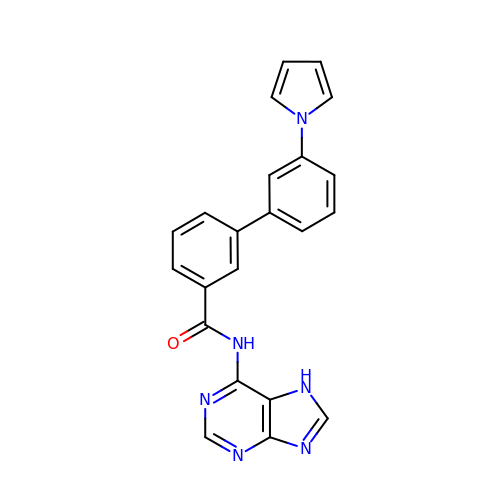~{N}-(7~{H}-purin-6-yl)-3-(3-pyrrol-1-ylphenyl)benzamide | C22 H16 N6 O | VPRBXPQTUPUOMQ-UHFFFAOYSA-N> MKVNNTIVVSIGQAGNQIAASFWKTVCLEHGIDPLTG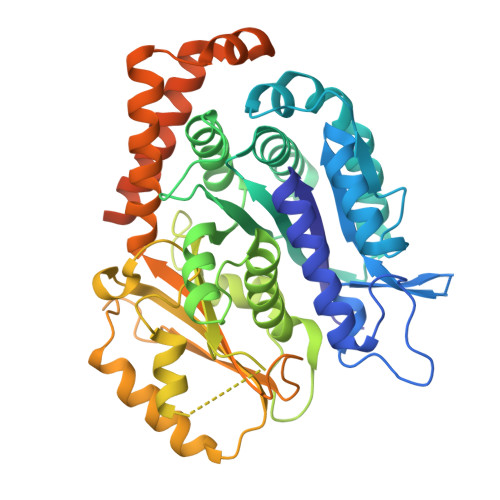QTAPGVAPRGNWSSFFSKLGESSSGSYVPRAIMVDLEPSVIDNVKATSGSLFNPANLISRTEGAGGNFAVGYLGAGREVLPEVMSRLDYEIDKCDNVGGIIVLHAIGGGTGSGFGALLIESLKEKYGEIPVLSCAVLPSPQVSSVVTEPYNTVFALNTLRRSADACLIFDNEALFDLAHRKWNIESPTVDDLNLLITEALAGITASMRFSGFLTVEISLRELLTNLVPQPSLHFLMCAFAPLTPPDGSDGEELGIEEMIKSLFDNGSVFAACSPMEGRFLSTAVLYRGIMEDKPLADAALAAMREKLPLTYWIPTAFKIGYVEQPGISHRKSMVLLANNTEIARVLDRICHNFDKLWQRKAFANWYLNEGMSEEQINVLRASAQELVQSYQVAEESGAKAKVQDSAGDTGMRAAAAGVSDDARGSMSLRDLVDRRR> MSPILGYWKIKGLVQPTRLLLEYLEEKYEEHLYERDEGDKWRNKKFELGLEFPNLPYYIDGDVKLTQSMAIIRYIADKHNMLGGCPKERAEISMLEGAVLDIRYGVSRIAYSKDFETLKVDFLSKLPEMLKMFEDRLCHKTYLNGDHVTHPDFMLYDALDVVLYMDPMCLDAFPKLVCFKKRIEAIPQIDKYLKSSKYIAWPLQGW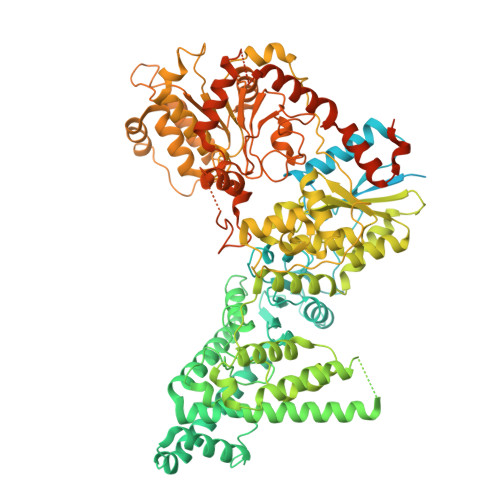QATFGGGDHPPKSDLEVLFQGPGSMTKIYLLTAPFDEEAKTGDGQYAASLELGFAENYEHIPCKWLKKDKGDYSIPFPTGTTSIPEETIPSAIVLQPVANENTVISGYKLKDTVSSPEKAQEVNNKTVSPRTPKIIVKHDNSLQSLTIMDIYSQKPIQFDESKVDEIIHSLETKKVNLEKAIEDNNAELSKIKKQKSKLAYLTRLYKENKENIQDYCTLNEYIEAHLFNPKFLSRHEKALNNFKALKSQFTGPVNLKELEKLTDKLTGIKEYSYDFHSNSLPYDLEHDKSFRNFYDFDGLKESIESIIKELEVLNSIRQAVSDKYPNSFKALNETEEHDDKLKFINIIFNDGFSTTYDQQTFIKALSALDIEKAIDAYTNVKNKLENTQDIIANKEGCRNKLISELQTLIANKQEPYLSANEKLGGFYSKRKLSASEGFHLAYQANRRDPIKPEVIENIITKMKPIDEDTHLDIHIRPPDCGVFITPEDIKKFQEAGIKVNITIHEYKQNYTRRYLQQYTHDLMRQANSVQFFNAEDRENAIIAATYGDCDKRNTTEPTGVAKKIREVGEDFDLDKYPVQKYDLKGKSGLTVASQKLSTEPDHPLDVVAKAPNILSFGTIRPGKGFEEALKLAQLIKDNSLSIHEKIKRVPIVKLAGDPQDKALMKQIVVERFGKTAVKTYQKTHPYDNRFNNSQRRDYWKNLVRELNAKVKEEVAVLNNPYIEIYPWCEPHELLDLKQNCKYVCRMDDMGMRNNGSAIISVLDVGVVYTKFGSVTDDIFIKGGKYGNAVDIGEYRYGKYSLLKKEKEFKEQHEEEPLPKWLIKNPDSAYKRQSESRDPKDILDSIVAREENQLICDNIEDSDNYRTVVEAQKLLKERFTLKNAVDHLLENIGLGHLIAQEEVDELFETVDPVQAQIDNLDILSDIKTPRLCLSRSCPELGFFGSRRGDLEAKQENNKLKESILVF> LDYHAC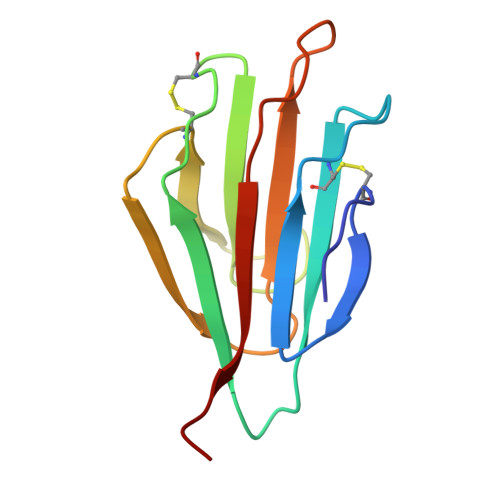GGRLTDDYGTIFTYKGPKTECVWTLQVDPKYKLLVSIPTLNLTCGKEYVEVLEGAPGSKSLGKFCEGLSILNRGSSGMTVKYKRDSGHPASPYEIIFLRDSQG> MNIIAIMGPHGVFYKDEPIKELESALVAQGFQIIWPQNSVDLLKFIEHNPRICGVIFDWDEYSLDLCSDINQLNEYLPLYAFINTHSTMDVSVQDMRMALWFFEYALGQAEDIAIRMRQYTDEYLDNITPPFTKALFTYVKERKYTFCTPGHMGGTAYQKSPVGCLFYDFFGGNTLKADVSISVTELGSLLDHTGPHLEAEEYIARTFGAEQSYIVTNGTSTSNKIVGMYAAPSGSTLLIDRNCHKSLAHLLMMNDVVPVWLKPTRNALGILGGIPRREFTRDSIEEKVAATTQAQWPVHAVITNSTYDGLLYNTDWIKQTLDVPSIHFDSAWVPYTHFHPIYQGKSGMSGERVAGKVIFETQSTHKMLAALSQASLIHIKGEYDEEAFNEAFMMHTTTSPSYPIVASVETAAAMLRGNPGKRLINRSVERALHFRKEVQRLREESDGWFFDIWQPPQVDEAECWPVAPGEQWHGFNDADADHMFLDPVKVTILTPGMDEQGNMSEEGIPAALVAKFLDERGIVVEKTGPYNLLFLFSIGIDKTKAMGLLRGLTEFKRSYDLNLRIKNMLPDLYAEDPDFYRNMRIQDLAQGIHKLIRKHDLPGLMLRAFDTLPEMIMTPHQAWQRQIKGEVETIALEQLVGRVSANMILPYPPGVPLLMPGEMLTKESRTVLDFLLMLCSVGQHYPGFETDIHGAKQDEDGVYRVRVLK

extracellular pH, and works in conjunction with a cognate inner membrane antiporter. excreted by the antiporter in exchange for a new amino acid substrate. that it is a decamer made of two pentameric rings. central pore, with the CTDs at the periphery.

for the polyamine production at neutral pH. decarboxylases have a similar enzymatic activity. between the inducible and the constitutive lysine decarboxylases. interacted with LdcI but was not capable of binding to LdcC. abolished by this procedure and no LdcIC-RavA complex could be detected. led to an assembly of the LdcCI-RavA complex.> MRRAAMYEEGPPPSYESVVSAAPVAAALGSPFDAPLDPPFVPPRYLRPTGGRNSIRYSELAPLFDTTRVYLVDNKSTDVASLNYQNDHSNFLTTVIQNNDYSPGEASTQTINLDDRSHWGGDLKTILHTNMPNVNEFMFTNKFKARVMVSRLPTKDNQVELKYEWVEFTLPEGNYSETMTIDLMNNAIVEHYLKVGRQNGVLESDIGVKFDTRNFRLGFDPVTGLVMPGVYTNEAFHPDIILLPGCGVDFTHSRLSNLLGIRKRQPFQEGFRITYDDLEGGNIPALLDVDAYQASLKDDTEQGGGGAGGSNSSGSGAEENSNA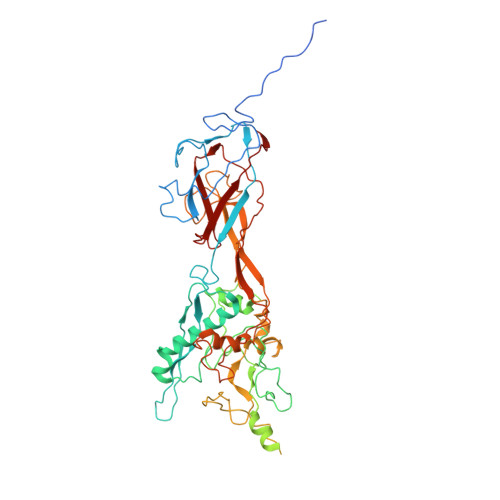AAAAMQPVEDMNDHAIRGDTFATRAEEKRAEAEAAAEAAAPAAQPEVEKPQKKPVIKPLTEDSKKRSYNLISNDSTFTQYRSWYLAYNYGDPQTGIRSWTLLCTPDVTCGSEQVYWSLPDMMQDPVTFRSTRQISNFPVVGAELLPVHSKSFYNDQAVYSQLIRQFTSLTHVFNRFPENQILARPPAPTITTVSENVPALTDHGTLPLRNSIGGVQRVTITDARRRTCPYVYKALGIVSPRVLSSRTF> PIPEQIKLIVDKWNPNHPNCAFKTYLYNKVDEHTVPLYGPGPNEDPK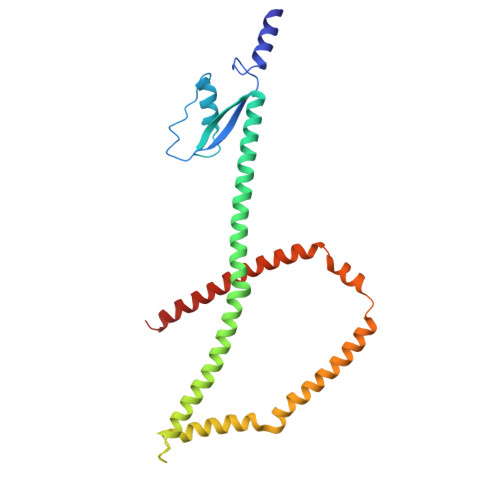EWEEALQRKPAPNFIPVLCSGFPSIVARLMLQRRVITEFNNKLHQINASLDAILSRHDLDHTVRAFNARRRHAELSRRCLHLAARVQVLRNRGYALSGDEDELKQKLQQIDKTLNDPAQGSRLEELWSRLIVLRGYAEDLKDQINQAGITESDGLGEEIEAKAKKILEDYDKQLQHLKKQVEEAKKDFEEWEKQ>[2x]FTSPAVKRLLGWKQGDEEEKWAEKAVDALVKKLKKKKGAMEELEKALSCPGQPSNCVTIPRSLDGRLQVSHRKGLPHVIYCRVWRWPDLQSHHELKPLECCEF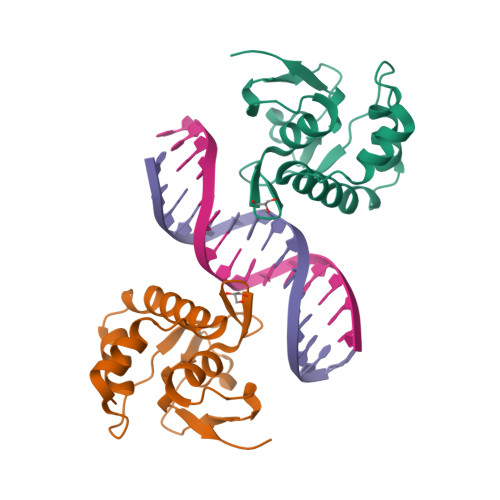PFGSKQKEVCINPYHYKRVES>GKITFFEDRSFQGRCYECSSDCPNLQTYFSRCNSVRVDSGCWMLYERPNYQGHQYFLRRGEYPDYQQWMGFSDSIRSCRLIPHAGSHRMRLYEKEDHKGVMMELSEDCSCIQDRFHLSEVRSLQVLEGCWVLYEMPNYRGRQYLLRPQEY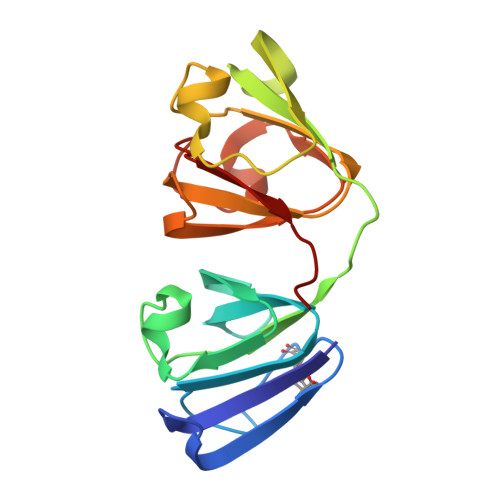RRFQDWGSVDAKAGSLRRVVDLY[2x]> SSFQSTVDSDSADQKEYLISDTGGQQLSISDAFIKESLFNRRVEEKSKELPFTPLGWHHNNLELLREENGEKQAMERLLSANHNHMMALLQQLLHSDSLSSSWRDIIVSLVCQVVQTVRPDVKNQDDDMDIRQFVHIKKIPGGKKFDSVVVNGFV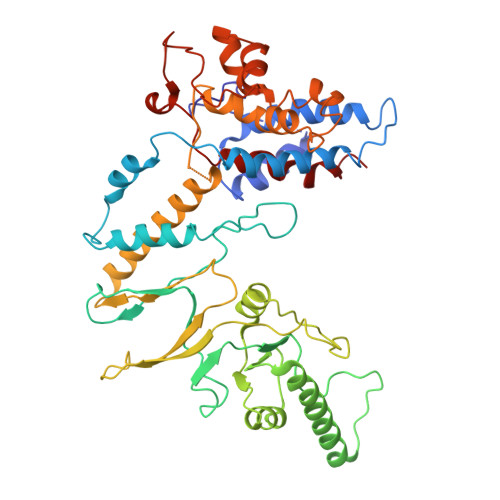CTKNIAHKKMSSCIKNPKILLLKCSIEYLYREETKFTCIDPIVLQEREFLKNYVQRIVDVRPTLVLVEKTVSRIAQDMLLEHGITLVINVKSQVLERISRMTQGDLVMSMDQLLTKPHLGTCHKFYMQIFQLPNEQTKTLMFFEGCPQHLGCTIKLRGGSDYELARVKEILIFMICVAYHSQLEISFLMDEFAMPPTLMQNPSFHSLIEGRGHEGAVQEQYGGGSIPWDPDIPPESLPCDDSSLLELRIVFEKGEQENKNLPQAVASVKHQEHSTTACPAGLPCAFFAPVPESLLPLP9-(4-azidobutyl)-8-bromanyl-purin-6-amine 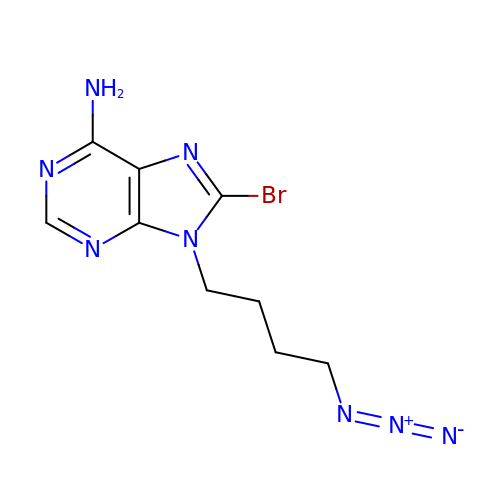| C9 H11 Br N8 | UOIUSKVGBLVETF-UHFFFAOYSA-N>[2x]MKPILVVGGGPAGLAATHALANVGQPSVLVEKRDRLGGAPIFSGYAKLVPSGRWANEAIGGMVSRIETDSLISIKTNTTVVSFDGDPNNFTAKLSDGTSIDCASAILTTGFSHFDSVNKPEWGFGMFPDVVTTTQVEQMISSGKGVRCLSDGRKPKRVAILLCVGSRDRQIGRE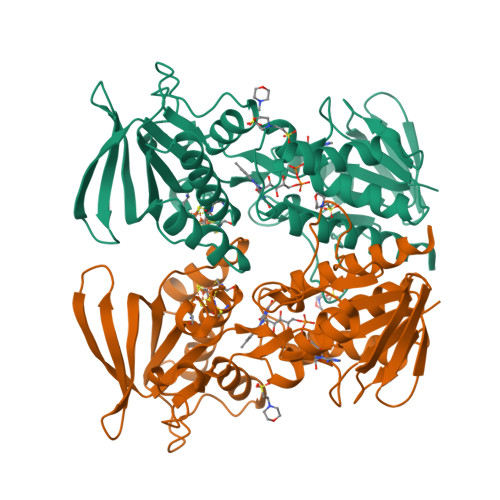WCSKICCTVSANLAMEIREELPDCHVYIYYMDIRTFGHYESDYYWRSQEEFKVKYIKARIAEVTSDGKQLIVKGEDTLVKRPITIPFDMVVHAIGMDPNVDNMTISAIFGVELHKHGYIARKDTYGLMGATSRPGVFVAGSAIGPETIDDSIAQANAAAMSALSLGRSIPREAAE>INHGYPIDPVPFTSVKVTDNFWGQRLQASREVTIPLAFSKCEETGRYENFVKAAHPSDTYKVEGFSFDDTDVYKTIEGASYSLQTYPDKKLQKYIDSVLVIVAGAQEPDGYLYTARTMNPKHPHNWAGKERWVAVENLSHEFYNLGHMIEGAVAHYQATGKRNFLDIAIKYADCVCREIGNGPQQKKYVPGHQIAEMALVKLYMATGDKKYLDQAKFFLDTRGYTSRKDTYSQAHKPVVEQDEAVGHAVRAVYMYSGMADVAAITGDSSYIKAIDKIWDNIVSKKIYITGGIGAHHAGEAFGNNYELPNLSAYCETCAAIGNVYMNYRLFLLHGDAKYFDVLERTLYNGLISGVSLDGGSFFYPNPLSSNGKYSRKPWFGCACCPSNVSRFIPSLPGYVYAVKNDQVYVNLYLSNKAELKVDKKKILLEQETGYPWNGDIRLKITQGNQDFTMKLRIPGWVRGNVLPGDLYSYADNQKPAYQVSVNGQTVESDVNDGYLSIARKWKKGDVVEVHFDMIPRIVKANPKVEADHGRVAVERGPIVYCAEWPDNRFNVHSILLNQHPQFKVTDKPELLYGIRQITTDAQALSYDKAGKLVTKDVELTLIPYYAWAHRGEGDMEVWLPIDVSATSAQ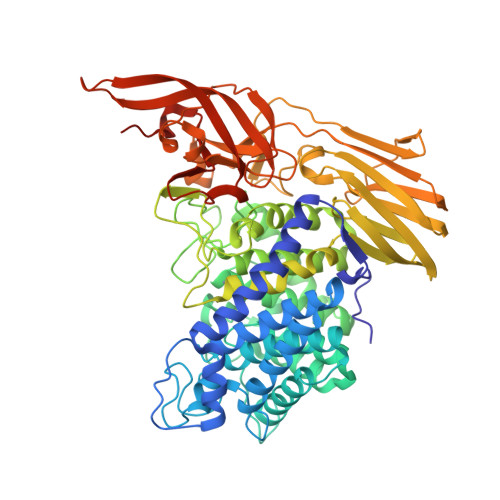PQEAGKWEDNGFFKN[2x]> MDLATLLGLIGGFAFVIMAMVLGGSIGMFVDVTSILIVVGGSIFVVLMKFTMGQFFGATKIAGKAFMFKADEPEDLIAKIVEMADAARKGGFLALEEMEINNTFMQKGIDLLVDGHDADVVRAALKKDIALTDERHTQGTGVFRAFGDVAPAMGMIGTLVGLVAMLSNMDDPKAIGPAMAVALLTTLYGAILSNMVFFPIADKLSLRRDQETLNRRLIMDGVLAIQDGQNPRVID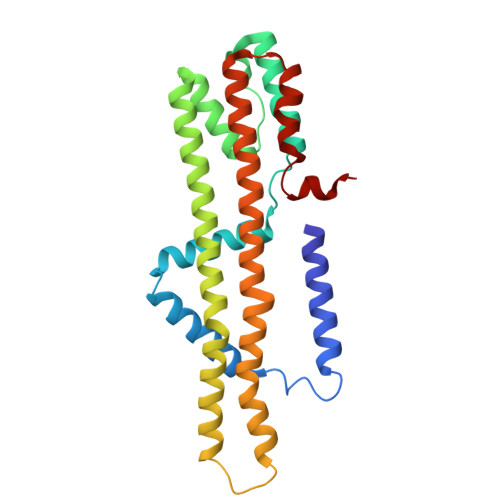SYLKNYLNEGKRALEIDE> GEMDERLLQKYRAQVFEWGGCFDKMFEALKSLIYLSEFENSEFDDEERHLLTLCIKHKISDYRTMTSQVLQEQTKQLNNDELVKICSEYVFSLRKDIKAFLQSFEDCVDRLVEKSFFSKFFKLKVKSDISRYKLEFGLCSLEDSKKIHQDAFTLLCEHPDKIEQLPLGFIQNLAYILSEKYG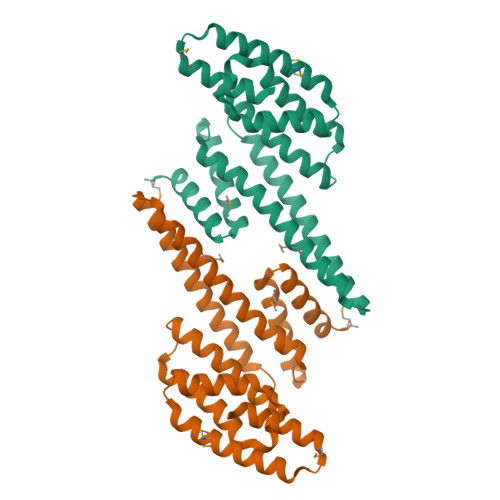EKKQVFNMLNSLGKILELQIKEQENMDRKAQITVYLQGIKDYIEK> MEQSSLLLKKQLADMRRVPVDGFSAGLVDDNDIYKWEVLVIGPPDTLYEGGFFKAILDFPRDYPQKPPKMKFISEIWHPNIDKEGNVCISILHDPGDDKWGYERPEERWLPVHTVETILLSVISMLTDPNFESPANVDAAKMQ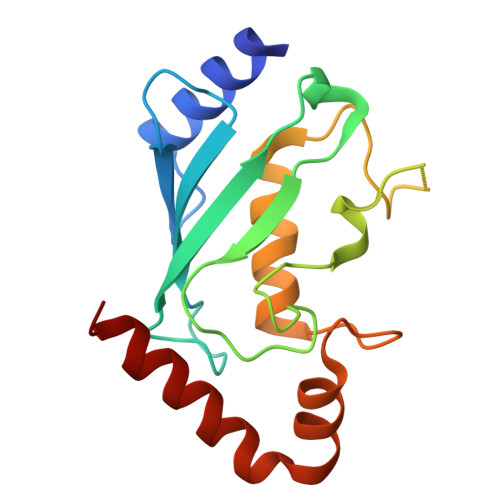RENYAEFKKKVAQCVRRSQEE>[4x]SVSPVEIAINP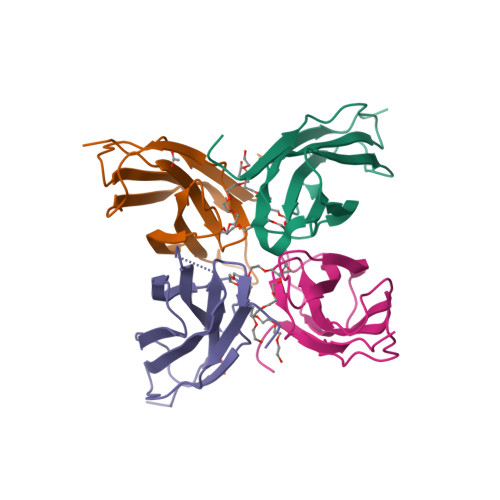ASEITATSAFISGTVTKFEQSKGFYGSGCNISLLYWEASNPMHVKVASSISKKDFPADISATIKDLKPHTTYQFKVTVNFYFSSSLQTFKTLAL> MNPVNATALYISASRLVLNYDPGDPKAFTEINRLLPYFRQSLSCCVCGHLLQDPIAPTNSTCQHYVCKTCKGKKMMMKPSCSWCKDYEQF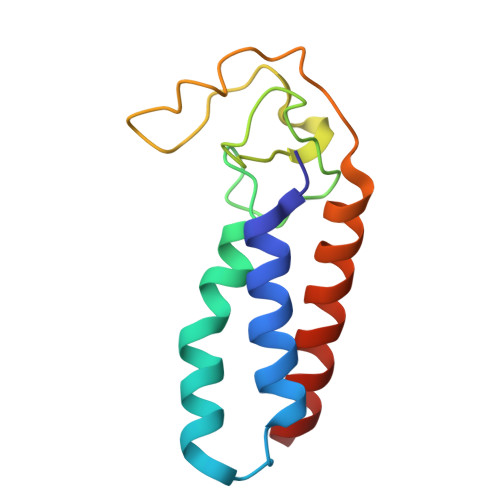EENKQLSILVNCYKKLCEYITQTTLA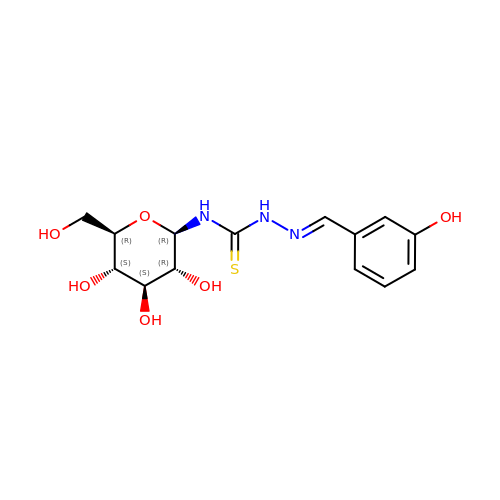N-({(2Z)-2-[(3-hydroxyphenyl)methylidene]hydrazino}carbonothioyl)-beta-D-glucopyranosylamine | C14 H19 N3 O6 S | FGOQDTKKNPWEBN-ARDSGTFASA-N>MMEFWGIEIKPGKPFKVIQKDGFMVHASQVTLGDVEKVKKDETFAVYVKIGDDENGFMIGNLSQKFPQFSIDLYLGHEFEISHNSTSSVYLIGYRTFDLEHH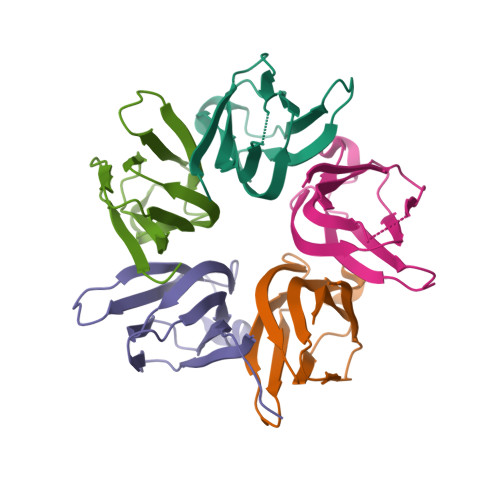H[5x]>MHHHHHHGGGGGMPASFERKLITRDALAAMRASLPAPVVFTNGVFDILHRGHVSYLADAKALGACLIVGVNSDASVRMLGKGDDRPINVQEDRMALLAALECVDWVVGFDEKTPVSLIEAVHPDILVKGGDYDMDALPESALVRGWGGRALAIPFEHDRS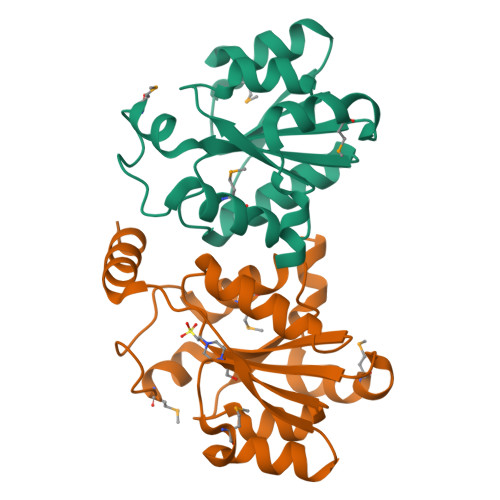TTALLKKVRAQSR[8x]> ACAMLERAKVKDEWAKAYGIGAARSKFGDALWRNVFNYAPNARDIFESVNSKDMASPEFKA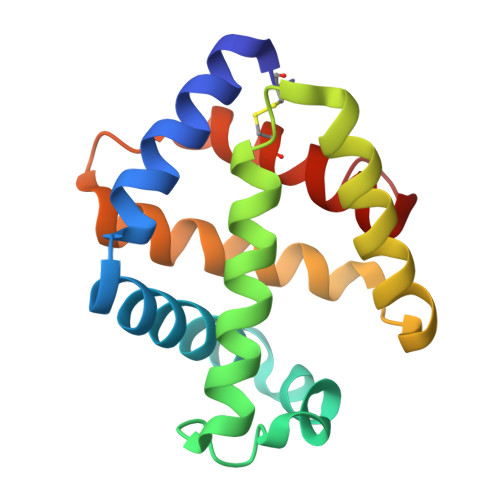HIARVLGGLDRVISMLDNQATLDADLAHLKSQHDPRTIDPVNFVVFRKALIATVAGTFGVCFDVPAWQGCYNIIAKGITGSDAA> AGFQLNEFSSSGLGRAYSGEGAIADDAGNVSRNPALITMFDRPTFSAGAVYIDPDVNISGTSPSGRSLKADNIAPTAWVPNMHFVAPINDQFG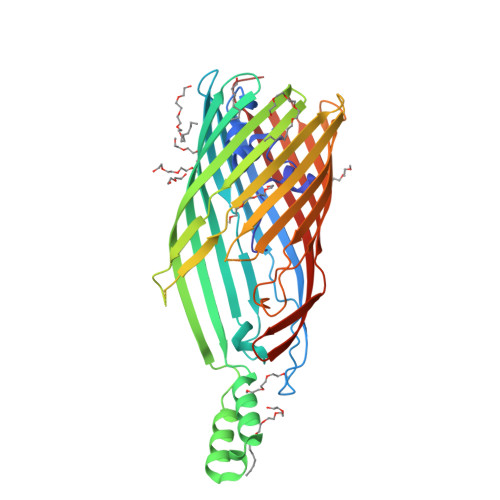WGASITSNYGLATEFNDTYAGGSVGGTTDLETMNLNLSGAYRLNNAWSFGLGFNAVYARAKIERFAGDLGQLVAGQIMQSPAGQTQQGQALAATANGIDSNTKTAHLNGNQWGFGWNAGILYELDKNNRYALTYRSEVKIDFKGNYSSDLNRAFNNYGLPIPTATGGATQSGYLTLNLPEMWEVSGYNRVDPQWAIHYSLAYTSWSQFQQLKATSTSGDTLFQKHEGFKDAYRIALGTTYYYDDNWTFRTGIAFRDSPVPAQNRSISIPDQDRFWLSAGTTYAFNKDASVDVGVSYMHGQSVKINEGPYQFESEGKAWLFGTNFNYAFHHHHHH>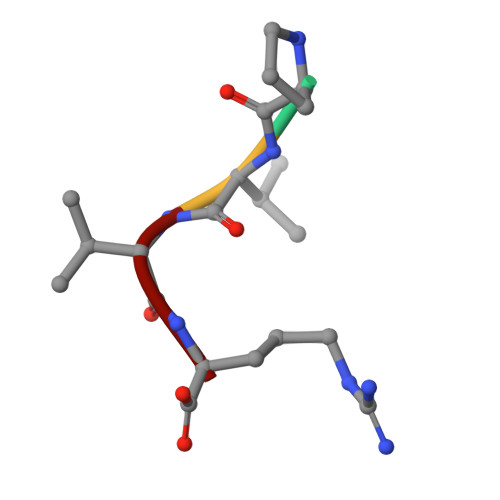 PVVR3-{5-[AMINO(IMINIO)METHYL]-6-CHLORO-1H-BENZIMIDAZOL-2-YL}-1,1'-BIPHENYL-2-OLATE 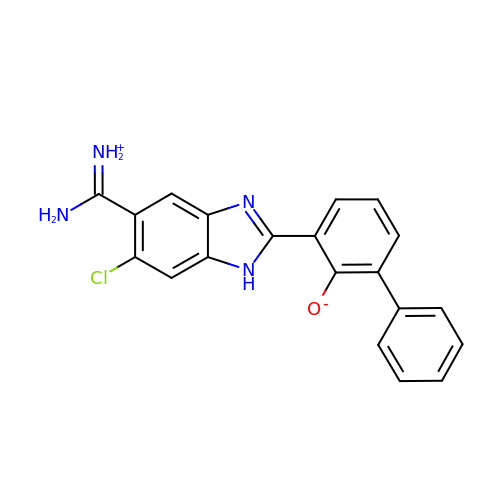| C20 H15 Cl N4 O | RPGVMAPDADAHPV-UHFFFAOYSA-N> XPK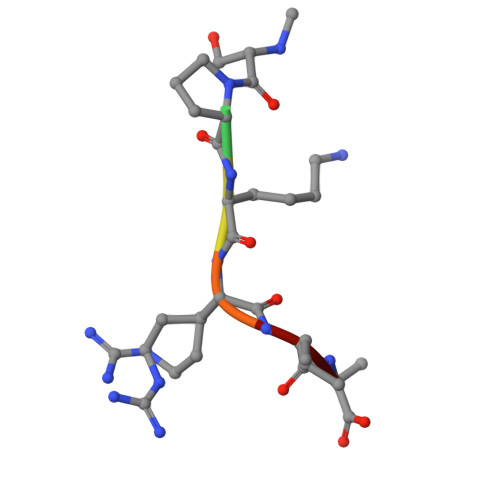RIA> GSNNQLVVRAKFNFQQTNEDELSFSKGDVIHVTRVEEG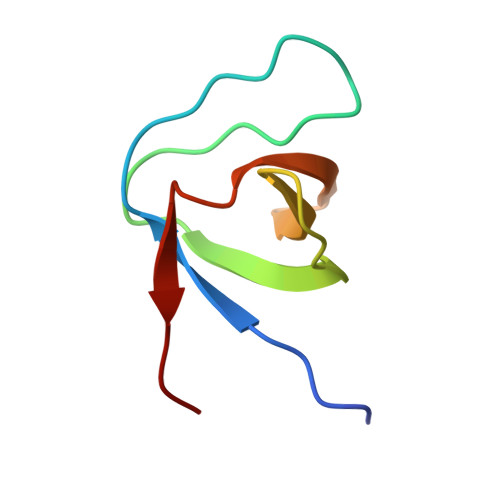GWWEGTLNGRTGWFPSNYVREVKA>RELYFQGMESVYLFSSGTLKRKANTICLETESGRKYIPVENVMDIKVFGEVDLNKRFLEFLSQKRIPIHFFNREGYYVGTFYPREYLNSGFLILKQAEHYINQEKRMLIAREIVSRSFQNMVDFLKKRKVRADSLTRYKKKAEEASNVSELMGIEGNAREEYYSMIDSLVSDERFRIEKRTRRPPKNFANTLISFGNSLLYTTVLSLIYQTHLDPRIGYLHETNFRRFSLNLDIAELFKPAVVDRLFLNLVNTRQINEKHFDEISEGLMLNDEGKSLFVKNYEQALRETVFHKKLNRYVSMRSLIKMELHKLEK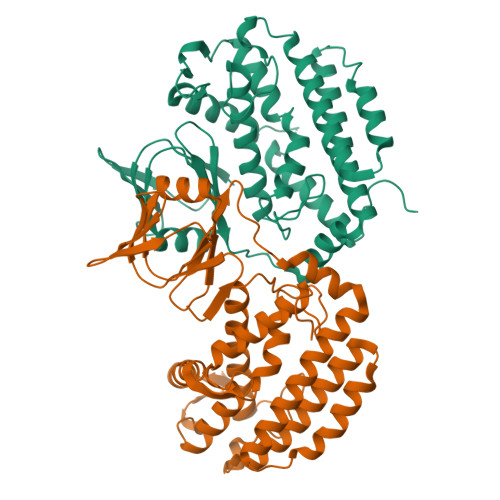HLIGEQVFGSEE[8x]> AQLTIEAVPSNAAEGKEVLLLVHNLPQDPRGYNWYKG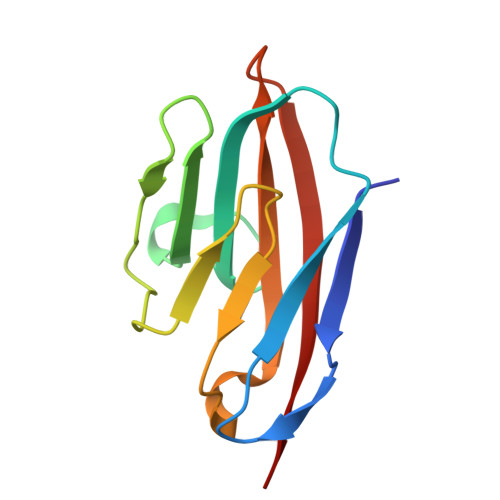ETVDANRRIIGYVISNQQITPGPAYSNRETIYPNASLLMRNVTRNDTGSYTLQVIKLNLMSEEVTGQFSVHC>SVAAHPWHDLEIGPGAPQIFNVVVEITKGSKVKYELDKKTGLIKVDRILYSSVVYPHNYGFVPRTLCEDNDPIDVLVIMQEPVLPGCFLRARAIGLMPMIDQGEKDDKIIAVCVDDPEYKHYTDIKELPPHRLSEIRRFFEDYKKNENKEVAVNDFLPSESAVEAIQYSMDLYAE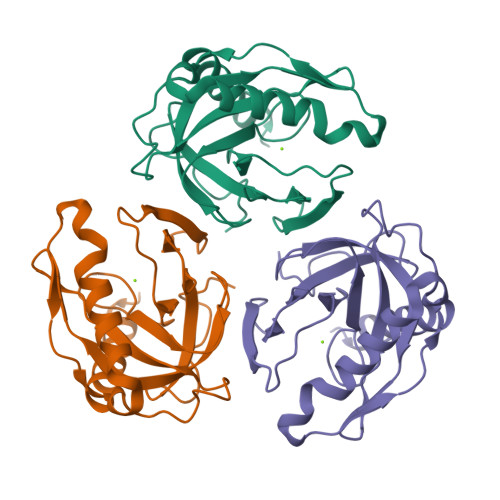YILH[2x]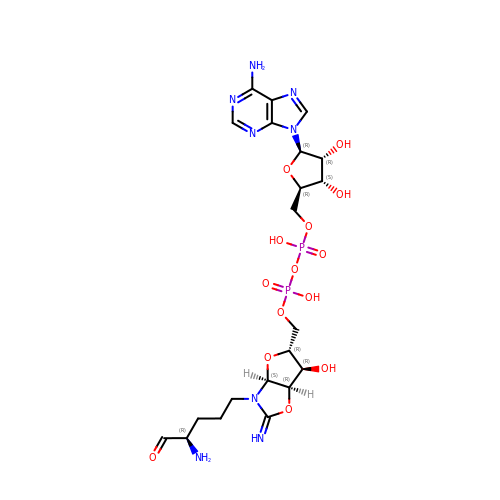[[(3~{a}~{S},5~{R},6~{R},6~{a}~{R})-2-azanylidene-3-[(4~{R})-4-azanyl-5-oxidanylidene-pentyl]-6-oxidanyl-3~{a},5,6,6~{a}-tetrahydrofuro[2,3-d][1,3]oxazol-5-yl]methoxy-oxidanyl-phosphoryl] [(2~{R},3~{S},4~{R},5~{R})-5-(6-aminopurin-9-yl)-3,4-bis(oxidanyl)oxolan-2-yl]methyl hydrogen phosphate | C21 H32 N8 O14 P2 | ZUWDPDYSBKPILX-IHCGFKTISA-N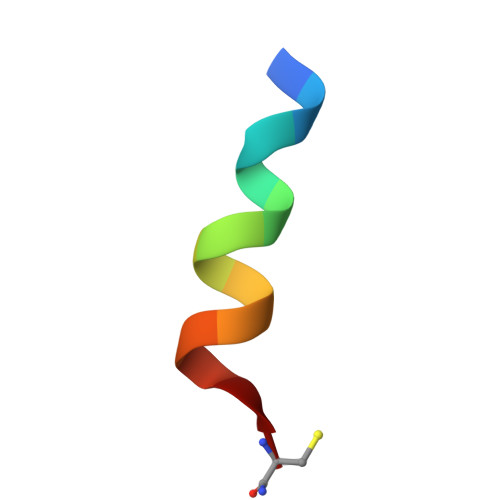> GPRLSRLLSAAGC> GPEKYKNILEKLEWYKNKSSEKYEFGIYEIDKREVFITTKYSYGFVNNKPLLPGHILLTTLKKKKHYNDLDIEEIIDINLLCNFMCYIMGNLFNTTDFSIAIQDGKEAGQTVDHVHIHIIPRKINDYKNNDNIYNDMNKINLGYGKNIICNSCNNTINVCSQNEIERNFKLEEFNTSIRSIEQMEEEANL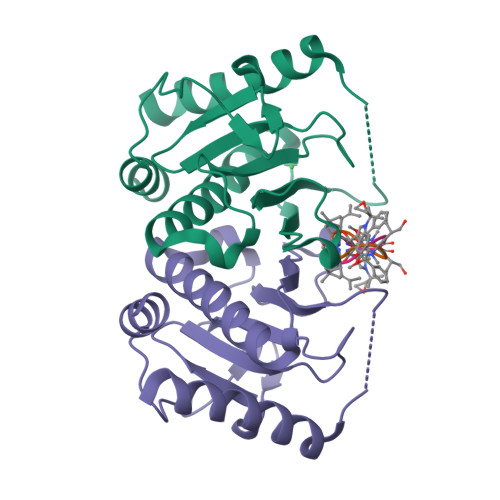IKSYINEKFSS;> WLAFVLV> MITPSIEYGLLSPMLIVFGVAIAGVLIEALAPRQSRYPLQVTLALGGLIATVVAVVFVARGLSGTPGRPAVLGAVVLDAPAVFLQGTIALVGILGIMLIAERQKATVSAGEARGLEDFTPQASAVAGSVAEQLATKTGVMQTEVFPLTMFAIGGMLLFPAADDLLTMFVALEVLSLPLYLLCGLARRRRLLSQEAALKYFLLGAFSSA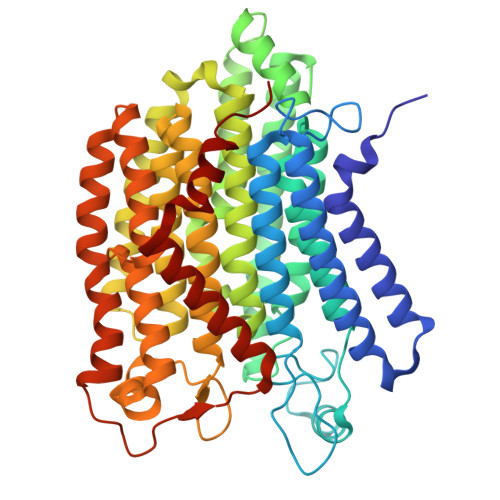FFIYGAAMLYGSAGTLDLSGIAESVAAGSGNTSLALLGVALLLVGVLFKVGAVPFHSWIPDVYQGAPTSITAFMAAATKIAAFGAMLRIFYVAVPALRDDWRPVLWAIAILTMVVGTVTAVTQTDVKRMLAYSAVAHSGFILTGVIAANPAGVSSTLFYLFAYGFSTLGAFAVVGLIRNAAGDEETSMAQWAGLGRRYPIVGVVFSLFLLAFAGIPLTSGFVSKFAVFKAAGEGGAIPLVIIGVIASAVAAYFYVRVIVLMFFTEPPDDAPELVVPSGLSTAVVTVTAAVTFALGALPQPLLDLANSAETFLH>GAMALPSGSDPAFSQPKSVLDAGLTCQGASPSSVSKPILLVPGTGTTGPQSFDSNWIPLSAQLGYTPCWISPPPFMLNDTQVNTEYMVNAITTLYAGSGNNKLPVLTWSQGGLVAQWGLTFFPSIRSKVDRLMAFAPDYKGTVLAGPLDALAVSAPSVWQLTTGSALTTALRNAGGLTQIVPTTNLYSATDEAVQPQVSNSPLDS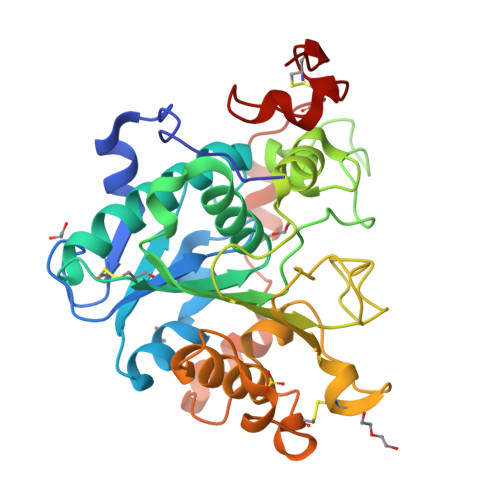SYLFNGKNVQAQAVCGPLFVIDHAGSLTSQFSYVVGRSALRSTTGQARSADYGITDCNPLPANDLTPEQKVAAAALLAPAAAAIVAGPKQNCEPDLMPYARPFAVGKRTCSGIVTP[2x]>GPDRSFRWKYHQFRFLCHSNALPSHVKISVSRQTLFEDSFQQIMNMKPYDLRRRLYIIMRGEEGLDYGGIAREWFFLLSHEVLNPMYCLFEYAGKNNYCLQINPASSINPDHLTYFRFIGRFIAMALYHGKFIDTGFTLPFYKRMLNKRPTLKDLESIDPEFYNSIVWIKENNLEECGLELYFIQDMEILGKVTTHELKEGGESIRVTEENKEEYIMLLTDWRFTRGVEEQTKAFLDGFNEVAPLEWLRYFDEKELELMLCGMQEIDMSDWQKSTIYRHYTKNSKQIQWFWQVVKEMDNEKRIRLLQFVTGTCRLPVGGFAELIGSNGPQKFCIDKVGKETWLPRSHTCFNRLDLPPYKSYEQLREKLLYAIEETE[2x];>XDPATIMCRAAADTCTFFX[2x]

Here, we report a general and rapid method for discovering α-helically constrained (Helicon) polypeptides that cooperatively induce the interaction between two target proteins without relying on previously known binders or an intrinsic affinity between the proteins. We show that Helicons are capable of binding every major class of E3 ubiquitin ligases, which are of great biological and therapeutic interest but remain largely intractable to targeting by small molecules. In addition to possessing increased stability and membrane permeability, Helicons are capable of binding large, flat protein surfaces that are inaccessible to targeting by small molecules, and Helicons have been developed to target a range of PPI targets in cells and in vivo. Characterizing Helicon-E3 co-structures and mechanisms of action, we identified new binding sites for α-helices on the E3 surfaces, as well as potential probes of the disease-linked E3, WWP123,24, highlighting the generality of our approach against this therapeutically important target class.

First, we focused on the NEDD4-like E3 ligases, which make up approximately a third of the HECT family. These include WWP1 and WWP2, which each consist of four tandem WW domains and a catalytic HECT domain at the C-terminus that transfers ubiquitin from a bound E2 first to itself and subsequently to the target substrate. Group 2 Helicons, the pan-HECT group including C73, bind both HECT domains, while Group 3 Helicons, the WWP2-HECT group including C72, bind only the WWP2 HECT domain (WWP2HECT). We next solved the crystal structures of five Helicons, four in complex with WWP2HECT representing all three groups of HECT-binding clusters, and one from Group 1 with WWP1HECT. These structures revealed three distinct Helicon binding sites on WWP2HECT. In all of the structures, we found that the HECT domains adopted similarly closed (inhibited) conformations. The WWP2 proteins in the co-structures with H301, H305, and H308 share a low root-mean-square deviation (RMSD = 0.5–0.8 Å) and are shown overlaid. Group 3 Helicon H305 binds a similar location near the interface of the N- and C-lobes of WWP2HECT, with binding residues predominantly in contact with the C-lobe. Consistent with their ability to impact the catalytic activity of WWP2HECT, H301 binds near the E2 interface, while H305 and H308 may restrict the conformational change involved in activating this domain. We found that individual Helicons from all three HECT-binding Groups (1–3) could modestly inhibit the auto-ubiquitylation activity of the isolated WWP2HECT.> MARRILVVEDEAPIREMVCFVLEQNGFQPVEAEDYDSAVNQLNEPWPDLILLAWMLPGGSGIQFIKHLR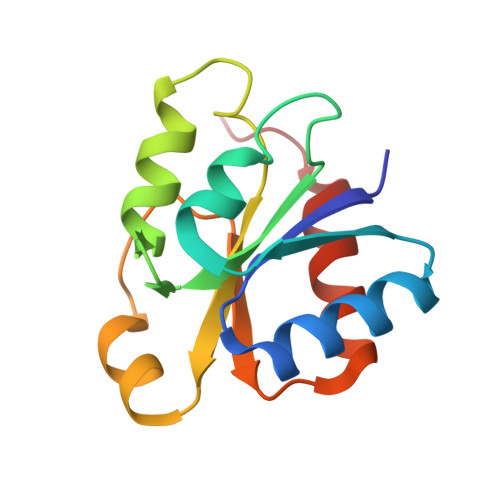RESMTRDIPVVMLTARGEEEDRVRGLETGADDCITKPFSPKELVARIKAVMRRISPMA>[2x]MRGSHHHHHHGSLATTLERIEKNFVITDPRLPDNPIIFASDSFLQLTEYSREEILGRNCRFLQGPETDRATVRKIRDAIDNQTEVTVQLINYTKSGKKFWNVFH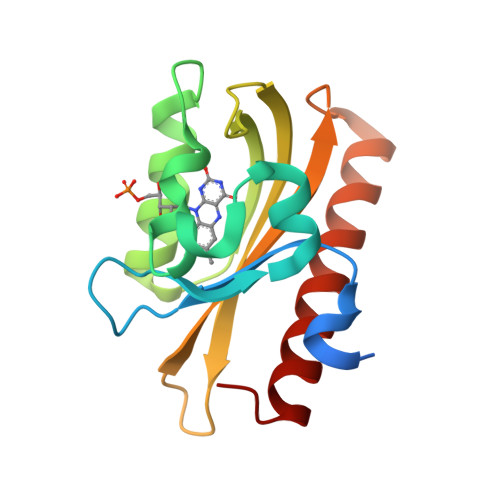LQPMRDYKGDVQYFIGVQLDGTERLHGAAEREAVCLIKKTAFQIAEAANDENYF>MAPPAVLSKSGVIYGKDVKDLFDYAQEKGFAIPAINVTSSSTVVAALEAARDNKAPIILQTSQGGAAYFAGKGVDNKDQAASIAGSIAAAHYIRAIAPTYGIPVVLHTDHCAKKLLPWFDGMLKADEEFFAKTGTPLFSSHMLDLSEETDDENIATCAKYFERMAKMGQWLEMEIGITGGEEDGVNNEHVEKDALYTSPETVFAVYESLHKISPNFSIAAAFGNVHGVYKPGNVQLRPEILGDHQVYAKKQIGTDAKHPLYLVFHGGSGSTQEEFNTAIKNGVVKVNLDTDCQYAYLTGIRDYVTNKIE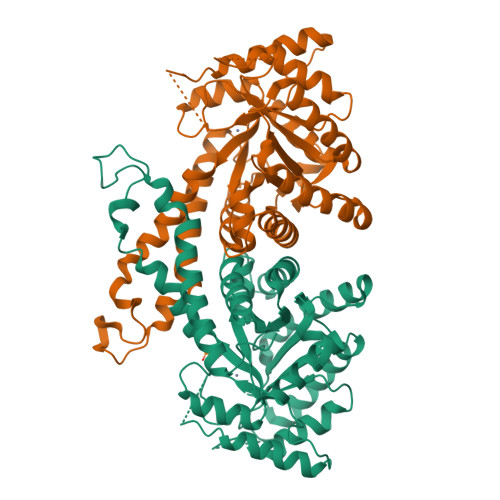YLKAPVGNPEGADKPNKKYFDPRVWVREGEKTMSKRIAEALDIFHTKGQLHHHHHH[2x]>MFSAGHKIKGTVVLMPKNELEVNPDGSAVDNLNAFLGRSVSLQLISATKADAHGKGKVGKDTFLEGINTSLPTLGAGESAFNIHFEWDGSMGIPGAFYIKNYMQVEFFLKSLTLEAISNQGTIRFVCNSWVYNTKLYKSVRIFFANHTYVPS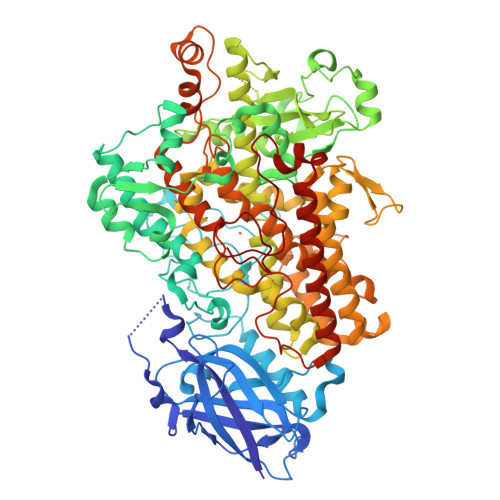ETPAPLVEYREEELKSLRGNGTGERKEYDRIYDYDVYNDLGNPDKSEKLARPVLGGSSTFPYPRRGRTGRGPTVTDPNTEKQGEVFYVPRDENLGHLKSKDALEIGTKSLSQIVQPAFESAFDLKSTPIEFHSFQDVHDLYEGGIKLPRDVISTIIPLPVIKELYRTDGQHILKFPQPHVVQVSQSAWMTDEEFAREMIAGVNPCVIRGLEEFPPKSNLDPAIYGDQSSKITADSLDLDGYTMDEALGSRRLFMLDYHDIFMPYVRQINQLNSAKTYATRTILFLREDGTLKPVAIELSLPHSAGDLSAAVSQVVLPAKEGVESTIWLLAKAYVIVNDSCYHQLMSHWLNTHAAMEPFVIATHRHLSVLHPIYKLLTPHYRNNMNINALARQSLINANGIGETTFLPSKYSVEMSSAVYKNWVFTDQALPADLIKRGVAIKDPSTPHGVRLLIEDYPYAADGLEIWAAIKTWVQEYVPLYYARDDDVKNDSELQHWWKEAVEKGHGDLKDKPWWPKLQTLEDLVEVCLIIIWIASALHAAVNFGQYPYGGLIMNRPTASRRLLPEKGTPEYEEMINNHEKAYLRTITSKLPTLISLSVIEILSTHASDEVYLGQRDNPHWTSDSKALQAFQKFGNKLKEIEEKLVRRNNDPSLQGNRLGPVQLPYTLLYPSSEEGLTFRGIPNSISI[2x]> MDSAITLWQFLLQLLQKPQNKHMICWTSNDGQFKLLQAEEVARLWGIRK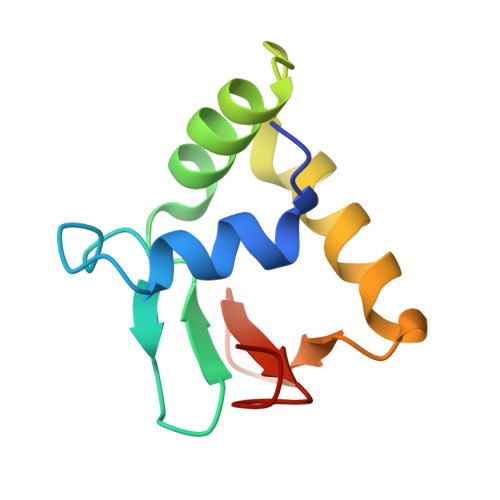NKPNMNYDKLSRALRYYYVKNIIKKVNGQKFVYKFVSYPEILNM> TGMDKSSIANKIEAYLGAKSDDSKIDQSLKADPSEVQYYGSGGDGYYLRKNICKITVNHSDSGTNDPCDRIPPPYGDNDQWKCAIILSKVSEKPENVFVPPRRQRMCINNLEKLNVDKIRDKHAFLADVLLTARNEGERIVQNHPDTNSSNVCNALERSFADIADIIRGTDLWKGTNSNLEQNLKQMFAKIRENDKVLQDKYPKDQNYRKLREDWWNANRQKVWEVITCGARSNDLLIKRGWRTSGKSNGDNKLELCRKCGHYEEKVPTKLDYVPQFLRWLTEWIEDFYREKQNLIDDMERHREECTSEDHKSKEGTSYCSTCKDKCKKYCECVKKWKSEWENQKNKYTELYQQNKNETSQKNTSRYDDYVKDFFKKLEANYSSLENYIKGDPYFAEYATKLSFILNSSDANNPSEKIQKNNDEVCNCNESGIASVEQEQISDPSSNKTCITHSSIKANKKKVCKHVKLGVRENDKDLRVCVIEHTSLSGVENCCCQDFLRILQENCSDNKSGSSSNGSCNNKNQEACEKNLEKVLASLTNCYKCDKCKSEQSKKNNKNWIWKKSSGKEGGLQKEYANTIGLPPRTQSLCLVVCLDEKGKKTQELKNIRTNSELLKEWIIAAFHEGKNLKPSHEKKNDDNGKKLCKALEYSFADYGDLIKGTSIWDNEYTKDLELNLQKIFGKLFRKYIKKNNTAEQDTSYSSLDELRESWWNTNKKYIWLAMKHGAGMNSTTCCGDGSVTGSGSSCDDIPTIDLIPQYLRFLQEWVEHFCKQRQEKVKPVIENCKSCKESGGTCNGECKTECKNKCEVYKKFIEDCKGGDGTAGSSWVKRWDQIYKRYSKYIEDAKRNRKAGTKNCGPSSTTNAAENKCVQSDIDSFFKHLIDIGLTTPSSYLSIVLDDNICGADKAPWTTYTTYTTTEKCNKETDKSKLQQCNTAVVVNVPSPLGNTPHGYKYACQCKIPTNEETCDDRKEYMNQWSCGSARTMKRGYKNDNYELCKYNGVDVKPTTVRSNSSKLDDKDVTFFNLFEQWNKEIQYQIEQYMTNTKISCNNEKNVLSRVSDEAAQPKFSDNERDRNSITHEDKNCKEKCKCYSLWIEKINDQWDKQKDNYNKFQRKQIYDANKGSQNKKVVSLSNFLFFSCWEEYIQKYFNGDWSKIKNIGSDTFEFLIKKCGNDSGDGETIFSEKLNNAEKKCKENESTNNKMKSSETSCDCSEPIYIRGCQPKIYDGKIFPGKGGEKQWICKDTIIHGDTNGACIPPRTQNLCVGELWDKRYGGRSNIKNDTKESLKQKIKNAIQKETELLYEYHDKGTAIISRNPMKGQKEKEEKNNDSNGLPKGFCHAVQRSFIDYKNMILGTSVNIYEYIGKLQEDIKKIIEKGTTKQNGKTVGSGAENVNAWWKGIEGEMWDAVRCAITKINKKQKKNGTFSIDECGIFPPTGNDEDQSVSWFKEWSEQFCIERLQYEKNIRDACTNNGQGDKIQGDCKRKCEEYKKYISEKKQEWDKQKTKYENKYVGKSASDLLKENYPECISANFDFIFNDNIEYKTYYPYGDYSSICSCEQVKYYEYNNAEKKNNKSLCHEKGNDRTWSKKYIKKLENGRTLEGVYVPPRRQQLCLYELFPIIIKNKNDITNAKKELLETLQIVAEREAYYLWKQYHAHNDTTYLAHKKACCAIRGSFYDLEDIIKGNDLVHDEYTKYIDSKLNEIFDSSNKNDIETKRARTDWWENEAIAVPNITGANKSDPKTIRQLVWDAMQSGVRKAIDEEKEKKKPNENFPPCMGVQHIGIAKPQFIRWLEEWTNEFCEKYTKYFEDMKSNCNLRKGADDCDDNSNIECKKACANYTNWLNPKRIEWNGMSNYYNKIYRKSNKESEDGKDYSMIMEPTVIDYLNKRCNGEINGNYICCSCKNIGENSTSGTVNKKLQKKETQCEDNKGPLDLMNKVLNKMDPKYSEHKMKCTEVYLEHVEEQLKEIDNAIKDYKLYPLDRCFDDKSKMKVCDLIGDAIGCKHKTKLDELDEWNDVDMRDPYNKYKGVLIPPRRRQLCFSRIVRGPANLRNLKEFKEEILKGAQSEGKFLGNYYNEDKDKEKALEAMKNSFYDYEYIIKGSDMLTNIQFKDIKRKLDRLLEKETNNTEKVDDWWETNKKSIWNAMLCGYKKSGNKIIDPSWCTIPTTETPPQFLRWIKEWGTNVCIQKEEHKEYVKSKCSNVTNLGAQESESKNCTSEIKKYQEWSRKRSIQWEAISEGYKKYKGMDEFKNTFKNIKEPDANEPNANEYLKKHCSKCPCGFNDMQEITKYTNIGNEAFKQIKEQVDIPAELEDVIYRLKHHEYDKGNDYICNKYK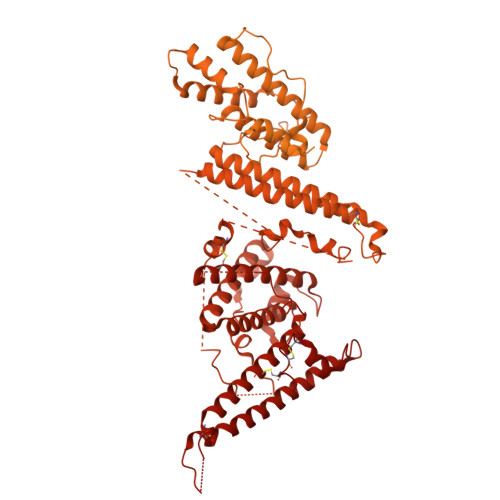NINVNMKKNNDDTWTDLVKNSSDINKGVLLPPRRKNLFLKIDESDICKYKRDPKLFKDFIYSSAISEVERLKKVYGEAKTKVVHAMKYSFADIGSIIKGDDMMENNSSDKIGKILGDGVGQNEKRKKWWDMNKYHIWESMLCGYKHAYGNISENDRKMLDIPNNDDEHQFLRWFQEWTENFCTKRNELYENMVTACNSAKCNTSNGSVDKKECTEACKNYSNFILIKKKEYQSLNSQYDMNYKETKAEKKESPEYFKDKCNGECSCLSEYFKDETRWKNPYETLDDTEVKNNCMCKPPPPASNNGTKHHHHHH>GANLERTFIAIKPDGVQRGLVGEIIKRFEQKGFRLVAMKFLRASEEHLKQHYIDLKDRPFFPGLVKYMNSGPVVAMVWEGLNVVKTGRVMLGETNPADSKPGTIRGDFCIQVGRNIIHGSDSVKSAEKEISLWFKPEELVDYKSCAHD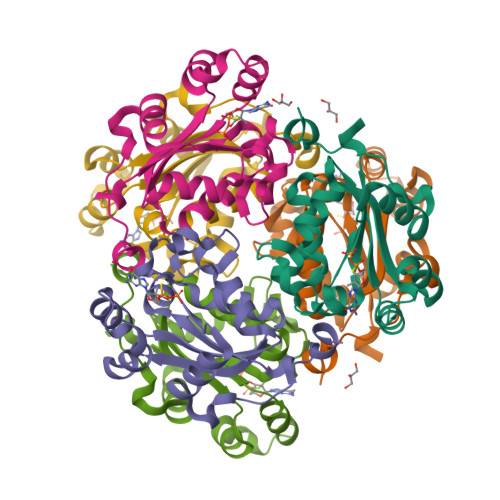WVYE[6x]> MSTQYETQGYTINNAGRRLVVDPITRIEGHMRCEVNINDQNVITNAVSCGTMFRGLEIILQGRDPRDAWAFVERICGVCTGVHALASVYAIEDAIGIKVPDNANIIRNIMLATLWCHAHLVHFYQLAGMDWIDVLDALKADPRKTSELAQSLSSWPKSSPGYFFDVQNRLKKFVEGGQLGIFRNGYWGHPQYKLPPEANLMGFAHYLEALDFQREIVKIHAVFGGKNPHPNWIVGGMPCAINIDESGAVGAVNMERLNLVQSIITRTADFINNVMIPDALAIGQFNKPWSEIGTGLSDKCVLSYGAFPDIANDFGEKSLLMPGGAVINGDFNNVLPVDLVDPQQVQEFVDHAWYRYPNDQVGRHPFDGITDPWYNPGDVKGSDTNIQQLNEQERYSWIKAPRWRGNAMEVGPLARTLIAYHKGDAATVESVDRMMSALNL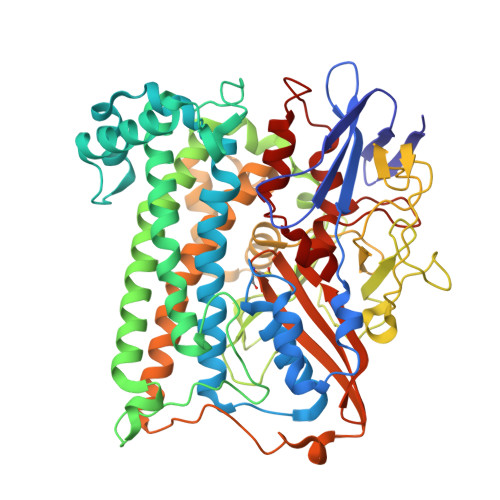PLSGIQSTLGRILCRAHEAQWAAGKLQYFFDKLMTNLKNGNLATASTEKWEPATWPTECRGVGFTEAPRGALGHWAAIRDGKIDLYQCVVPTTWNASPRDPKGQIGAYEAALMNTKMAIPEQPLEILRTLHSFDPCLACSTH> MILDTDYITEDGKPVIRIFKKENGEFKIEYDRTFEPYFYALLKDDSAIEEVKKITAERHGTVVTVKRVEKVQKKFLGRPVEVWKLYFTHPQDVPAIRDKIREHPAVIDIYEYDIPFAKRYLIDKGLVPMEGDEELKMLAFDIETLYHEGEEFAEGPILMISYADEEGARVITWKNVDLPYVDVVSTEREMIKRFLRVVKEKDPDVLITYNGDNFDFAYLKKRCEKLGINFALGRDGSEPKIQRMGDRFAVEVKGRIHFDLYPVIRRTINLPTYTLEAVYEAVFGQPKEKVYAEEITTAWETGENLERVARYSMEDAKVTYELGKEFLPMEAQLSRLIGQSLWDVSRSSTGNLVEWFLLRKAYERNELAPNKPDEKELARRRQSYEGGYVKEPERGLWENIVYLDFRSLYPSIIITHNVSPDTLNREGCKEYDVAPQVGHRFCKDFPGFIPSLLGDLLEERQKIKKKMKATIDPIERKLLDYRQRAIKILANSYYGYYGYARARWYCKECAESVTAWGREYITMTIKEIEEKYGFKVIYSDTDGFFATIPGADAETVKKKAMEFLKYINAKLPGALELEYEGFYKRGFFVTKKKYAVIDEEGKITTRGLEIVRRDWSEIAKETQARVLEALLKDGDVEKAVRIVKEVTEKLSKYEVPPEKLVIHEQITRDLKDYKATGPHVAVAKRLAARGVKIRPGTVISYIVLKGSGRIGDRAIPFDEFDPTKHKYDAEYYIENQVLPAVERILRAFGYRKEDLRYQKTRQVGLSAWL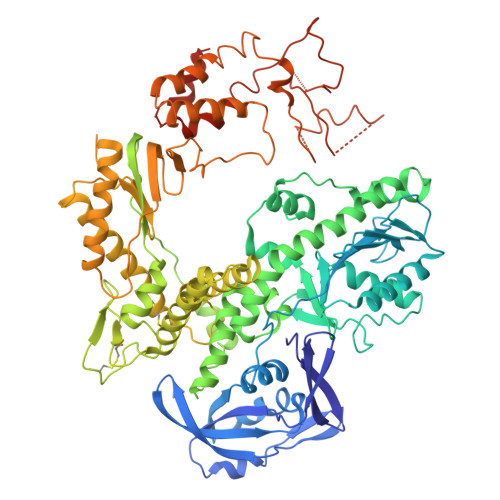KPKGT>GSSSGRQGGVHELSAFEQLVVELVRHDDSWPFLKLVSKIQVPDYYDIIKKPIALNIIREKVNKCEYKLASEFIDDIELMFSNCFEYNPRNTSEAKAGTRLQAFFHIQAQKLGLHVT[4x]

Near their C-termini BAZ1A and BAZ1B each contain a plant homeodomain (PHD) and a bromodomain (BD). Here, we use CRISPR-Cas9-mediated and lentiviral-mediated genome editing to reveal that the non-catalytic subunits BAZ1A and BAZ1B are key for recovery after DNA damage in human cells, in part by recruiting the ATPase SMARCA5 to damaged chromatin. Moreover, we report the crystal structure of BAZ1A-BD, and we discover the ability of BAZ1A-PHD to bind DNA. Our study reveals that the PHD and BD domains of BAZ1A each support BAZ1A cellular function through the non-canonical biochemical features discovered here.

The C-terminal regions of BAZ1A and BAZ1B each contain one BD of unknown function. Both BAZ1A-BD and BAZ1B-BD bear a conserved asparagine “anchor” residue that, in functional BDs, hydrogen bonds with the carbonyl group of a bound acyl-lysine ligand and is required for this interaction. However, the BAZ1A-BD gatekeeper is a non-canonical glutamic acid. We confirmed that this non-canonical feature is compatible with the BD fold by solving the crystal structure of BAZ1A-BD to 1.7 Å resolution. We could not detect BAZ1A-BD binding to any of the peptides on the array. To test whether the glutamic acid gatekeeper inhibits the binding of BAZ1A-BD to acetylated peptides, we replaced it with a valine like in BAZ1B-BD. Unlike the wild-type domain, BAZ1A-BDE1515V showed substantial binding to the array that was dependent on peptide acetylation. To test whether the weak binding of wild-type BAZ1A-BD to acetylated peptides was mediated by the canonical BD pocket, we replaced the asparagine anchor with a tyrosine residue (N1509Y; BDNY) to completely abrogate acetyl-lysine recognition. The binding signal for the BAZ1A-BDNY mutant was indistinguishable from background and that observed for wild-type and unmodified peptides. We conclude that, while the BDs of BAZ1A and BAZ1B are both compatible with canonical BD function, the presence of a glutamic acid at the gatekeeper position substantially lowers the binding affinity of BAZ1A-BD to acetylated histone peptides. Moreover, the complete elimination of acetyl-lysine recognition by removal of the asparagine anchor is highly detrimental to the function of BAZ1A in cells. Together, the data suggest that BAZ1A-BD has evolved to bind acetylated histones with a specific affinity, and either increasing or decreasing the affinity of this interaction prevents BAZ1A from functioning in DNA damage recovery.Type IA topoisomerases (TopoIAs) are present in all living organisms. They resolve DNA/RNA catenanes, knots and supercoils by breaking and rejoining single-stranded DNA/RNA segments and allowing the passage of another nucleic acid segment through the break. Topoisomerase III-β (TOP3B), the only RNA topoisomerase in metazoans, promotes R-loop disassembly and translation of mRNAs. We present a series of cryo-EM structures of human TOP3B with its cofactor TDRD3 during cleavage and rejoining of DNA or RNA, thus elucidating the roles of divalent metal ions and key enzyme residues in each step of the catalytic cycle.

To capture the strand passage event or the passing DNA in the large central cavity of the enzyme, we replaced the gapped 43-mer DNA substrate with a DNA bubble, in which the 11-nt ssDNA is opposite to 13 unmatched nucleotides. Additionally, we identified species with two cTOP3B bound to one DNA bubble and obtained a ~ 4.3 Å cryo-EM density map of this cTOP3B dimer from 63,000 particles. Within this complex, one enzyme binds to the 11-nt strand and forms a cleavage complex. The second enzyme binds to the opposite 13-nt strand without cleaving DNA. Remarkably, the second cTOP3B assumes an open-gate conformation with a dsDNA arm trapped in the gap between domains I and III and interacting with domains III and II via charged residues. Interactions between domains III of two TOP3B molecules provide additional stability to this open-gate conformation. While the closed cTOP3B exhibits a planar ring conformation, switching to the open conformation induces a major swing of domains II and III with rotation of domain III over 60° coupled with a ~ 40 Å translation that opens the planar ring. The catalytic tyrosine in domain III disengages from the MnC2+ binding site in domain I, creating a 40 Å gap between them, which may represent the open ssDNA gate of TOP3B in the DNA-cleaved state. This conformational transition also disassembles the hydrophobic core between domains III and IV, leaving only a weak charge interaction between them. In our resolved TOP3B dimer complex, the opening of one TOP3B is possibly driven by binding energy from interactions with both the DNA and the second TOP3B.

>[2x]VMKTVLMVAEKPSLAQSIAKILSRGSLSSHKGLNGACSVHEYTGTFAGQPVRFKMTSVCGHVMTLDFLGKYNKWDKVDPAELFSQAPTEKKEANPKLNMVKFLQVEGRGCDYIVLWLDCDKEGENICFEVLDAVLPVMNKAHGGEKTVFRARFSSITDTDICNAMACLGEPDHNEALSVDARQELDLRIGCAFTRFQTKYFQGKYGDLDSSLISFGPCQTPTLGFCVERHDKIQSFKPETYWVLQAKVNTDKDRSLLLDWDRVRVFDREIAQMFLNMTKLEKEAQVEATSRKEKAKQRPLALNTVEMLRVASSSLGMGPQHAMQTAERLYTQGYISYPRTETTHYPENFDLKGSLRQQANHPYWADTVKRLLAEGINRPRKGHDAGDHPPITPMKSATEAELGGDAWRLYEYITRHFIATVSHDCKYLQSTISFRIGPELFTCSGKTVLSPGFTEVMPWQSVPLEESLPTCQRGDAFPVGEVKMLEKQTNPPDYLTEAELITLMEKHGIGTDASIPVHINNICQRNYVTVESGRRLKPTNLGIVLVHGYYKIDAELVLPTIRSAVEKQLNLIAQGKADYRQVLGHTLDVFKRKFHYFVDSIAGMDELMEVSF;>[2x]MAQVAGAALSQAGWYLSDEGIEACTSSPDKVNVNDIILIALNTDLRTIGKKFLPSDINSGKVEKLEGPCVLQIQKIRNVAAPKDNEESQAAPRMLRLQMTDGHISCTAVEFSYMSKISLNTPPGTKVKLSGIVDIKNGFLLLNDSNTTVLGGEVEHLIEKW>GSHEEENDVVKGNFDISKISGDWYSILLASDIKEKIEENGSMRVFVKDIEVLSNSSLIFTMHTKVNGKCTKISLICNKTEKDGEYDVVHDGYNLFRIIETAYEDYIIFHLNNVNQEQEFQLMELYGRKPDVSPKVKEKFVRYCQGMEIPKENILDLTQVDRCLQARQSEAAQVSSAE[4x]

Can f 6, a recently identified lipocalin allergen produced from the submaxillary gland and detected in dander, shows a high amino acid sequence identity with Fel d 4 (67%) and Equ c 1 (55%), major cat and horse lipocalin allergens, respectively. Lipocalins are characterised by a common tertiary structure exhibiting an eight-stranded, antiparallel β-sheet closed back on itself forming a continuous hydrogen-bonded β-barrel.

In this study, we produced a recombinant protein of the dog lipocalin allergen Can f 6 (rCan f 6) and determined its three-dimensional structure at 2.35 Å resolution. rCan f 6 crystals diffracted to 2.35 Å resolution and the structure was refined to an R-factor of 20.3% and an Rfree of 26.9%. For the final model, four rCan f 6 molecules consisting of chains A to D were contained in an asymmetric unit and had nearly identical structures with an average root mean square deviation (RMSD) of 0.63 Å for main-chain atoms. Two regions with high RMSD, Leu50–Ser53 and Val111–Gln115, are located on the extruded turn and exposed to the solvent. For Leu50–Ser53, chain C exhibits an alternate conformation due to the lack of hydrogen bond(s) between the Oδ/Nδ atom(s) of Asn52 and Oγ atom of Ser54. The high RMSD at Val111–Gln115 reflects differences in packing environments among the four molecules. All other regions are superimposable among the four molecules in the asymmetric unit with low RMSD, indicating that the four molecules have essentially the same structures. The estimated molecular mass was 19.9 kDa, indicating that rCan f 6 is present as a monomer in solution. Hilger et al. modelled the tertiary structure of Can f 6 and Fel d 4 in silico based on the crystal structure of Equ c 1 and showed that these allergens share highly conserved structural characteristics as well as amino acid sequence identity. Consistent with these findings, the X-ray crystal structure characteristics of Can f 6 remarkably resembled those of Equ c 1.>[4x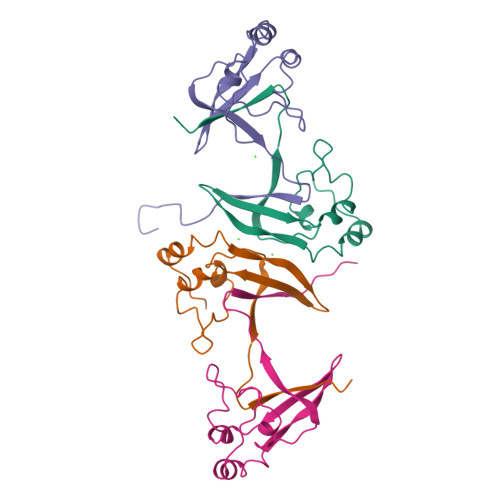]MSKSGVPRLLTASERERLEPFIDQIHYSPRYADDEYEYRHVMLPKAMLKAIPTDYFNPETGTLRILQEEEWRGLGITQSLGWEMYEVHVPEPHILLFKREKDYQMKSQQRGG PsaA is the solute-binding protein (SBP) of a manganese-specific ABC permease encoded by the psaBCA locus. Mn(II) acquisition, mediated by PsaA, is important for S. pneumoniae growth, proliferation and virulence. Intriguingly, both Mn(II) and Zn(II) are acquired by SBPs belonging to the Cluster A-1 family of prokaryotic transporters. Studies from our laboratory have previously demonstrated that the pneumococcal surface antigen A (PsaA) from S. pneumoniae has a clear interaction with Zn(II) despite not being involved in its uptake, which occurs via a distinct Zn(II) ATP-binding cassette (ABC) permease.

The crystal structure of PsaA had previously been determined with Zn(II) tetrahedrally coordinated by the four metal-binding residues (His67, His139, Glu205 and Asp280) but no structure for the Mn(II)-loaded protein has been reported. Well-defined and continuous electron density was observed for the active site residues that tetrahedrally coordinated the metal ion, which was identified as Mn(II) (see Text S2 for further details). The tetrahedral coordination of Mn(II) is analogous to Zn(II) coordination in PsaA and the structures of other Cluster A-1 SBPs (Treponema pallidum TroA, Synechocystis 6803 MntC, Synechocystis 6803 ZnuA and E. coli ZnuA). Overall, our structural analysis indicates that PsaA is capable of binding Mn(II) and Zn(II) with only very minor accompanying structural changes in the final loaded state. Metal ion discrimination within the Cluster A-1 SBPs is proposed to occur through subtle differences in the binding sites, Zn(II)-binding being favoured by the presence of three N ligands (from His residues), and Mn(II)-binding being favoured by two N (His) and two O (Asp or Glu) ligands. The derived affinity constants (1/KA = KD) calculated for 1∶1 complexes of PsaA with Mn(II) or Zn(II) were 3.3±1.0 nM and 231±1.9 nM, respectively. However, the preference of PsaA for Mn(II) is the result of the highly unfavourable entropic contribution of Zn(II) binding (−TΔS = 9.5±0.4 kcal.mol−1) relative to Mn(II) (−TΔS =  −4.0±0.9 kcal.mol−1). Here we show PsaA in complex with its physiological ligand and the difference in the affinities for Mn(II) and Zn(II) confirm its physiological role in Mn(II) acquisition. In contrast, the Mn(II)-PsaA complex likely represents a reversible complex that, upon interaction with the ABC permease, delivers the metal ion into the transporter and allows apo-PsaA to be released. Furthermore, consistent with the lack of solvent access to the binding site in the metal loaded-PsaA structures, we observed that Zn(II) could not be extracted from PsaA by chelating agents, despite the protein's lower affinity for the metal, or by competition with Mn(II).

>WRGSHHHHHHGSACASGKKDTTSGQKLKVVATNSIIADITKNIAGDKIDLHSIVPIGQDPHEYEPLPEDVKKTSEADLIFYNGINLETGGNAWFTKLVENAKKTENKDYFAVSDGVDVIYLEGQNEKGKEDPHAWLNLENGIIFAKNIAKQLSAKDPNNKEFYEKNLKEYTDKLDKLDKESKDKFNKIPAEKKLIVTSEGAFKYFSKAYGVPSAYIWEINTEEEGTPEQIKTLVEKLRQTKVPSLFVESSVDDRPMKTVSQDTNIPIYAQIFTDSIAEQGKEGDSYYSMMKYNLDKIAEGLAK[4x]> MEPHSLRYDFTVLSWDGSVQSGFLTEVHLDGQPFIRCDRQKCRAKPQGQWAEDVLGNKTWDRETRDLTGNGKDLRMTLAHIKDQKEGLHSLQEIRVCEIHEDNSTRSSHHFYYDGELFLSWNLETKEFTMPQSSRAQTLAMNVRNFWKEDAMKTKTHFHAMRADCLQELRRYLKSGVILRRTVPPMVNVTRSEASEGNITVTCRASGFYPWNITLSWRQDGVSLSHDT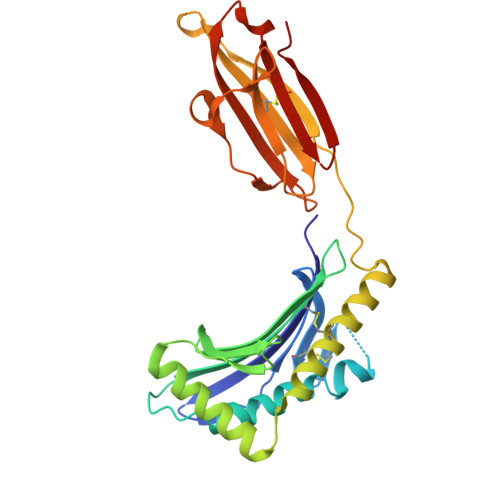QQWGDVLPDGNGTYQTWVATRICQGEEQRFTCYMEHSGNHSTHPVPS> MGSNPPASPLQDNLVIALHSYEPSHDGDLGFE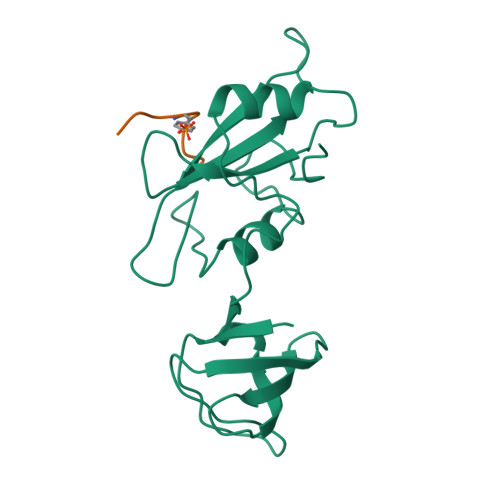KGEQLRILEQSGEWWKAQSLTTGQEGFIPFNFVAKANSLEPEPWFFKNLSRKDAERQLLAPGNTHGSFLIRESESTAGSFSLSVRDFDQNQGEVVKHYKIRNLDNGGFYISPRITFPGLHELVRHYTNASDGLCTRLSRPCQT;> EGQYQPQPA N'-hydroxy-N-phenyl-3-(trifluoromethyl)benzenecarboximidamide | C14 H11 F3 N2 O | 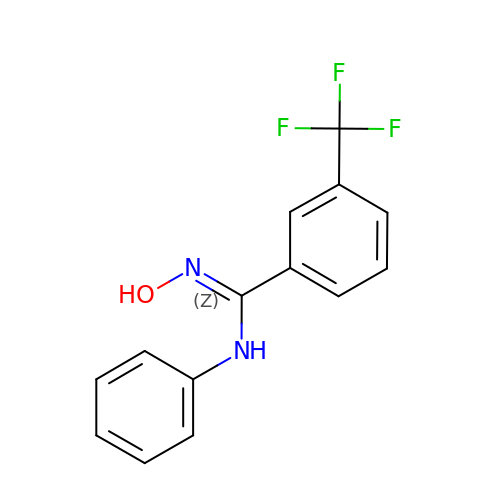SFPWZRCGYUTPNJ-UHFFFAOYSA-N>GSNRSLIVTTLLEEPFVMFRKSDRTLYGNDRFEGYCIDLLKELAHILGFSYEIRLVEDGKYGAQDDKGQWNGMVKELIDHKADLAVAPLTITHVREKAIDFSKPFMTLGVSILYRKGTPIDSADDLAKQTKIEYGAVKDGATMTFFKKSKISTFEKMWAFMSSKPSALVKNNEEGIQRTLTADYALLMESTTIEYI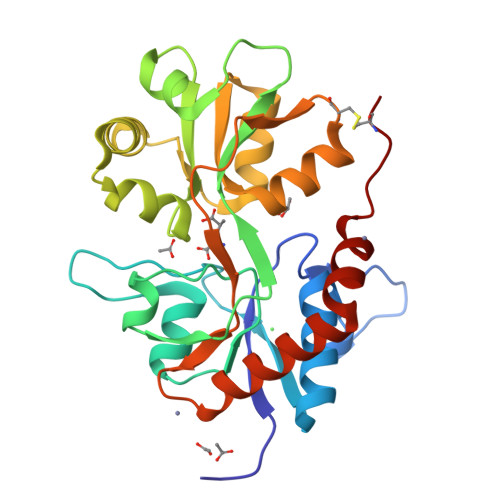TQRNCNLTQIGGLIDSKGYGIGTPMGSPYRDKITIAILQLQEEDKLHIMKEKWWRGSGCPE[2x]> MAQILPIRFQEHLQLQNLGINPANIGFSTLTMESDKFICIREKVGEQAQVVIIDMNDPSNPIRRPISADSAIMNPASKVIALKAGKTLQIFNIEMKSKMKAHTMTDDVTFWKWISLNTVALVTDNAVYHWSMEGESQPVKMFDRHSSLAGCQIINYRTDAKQKWLLLTGISAQQNRVVGAMQLYSVDRKVSQPIEGHAASFAQFKMEGNAEESTLFCFAVRGQAGGKLHIIEVGTPPTGNQPFPKKAVDVFFPPEAQNDFPVAMQISEKHDVVFLITKYGYIHLY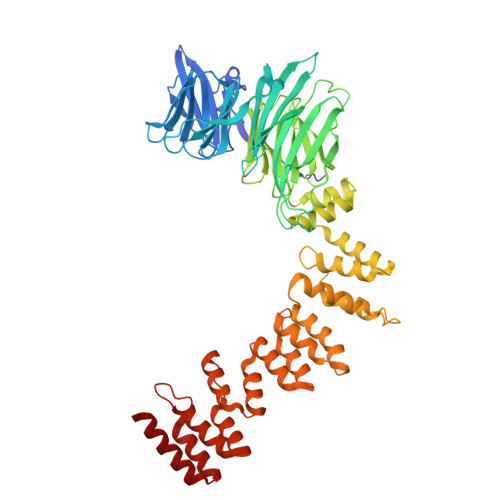DLETGTCIYMNRISGETIFVTAPHEATAGIIGVNRKGQVLSVCVEEENIIPYITNVLQNPDLALRMAVRNNLAGAEELFARKFNALFAQGNYSEAAKVAANAPKGILRTPDTIRRFQSVPAQPGQTSPLLQYFGILLDQGQLNKYESLELCRPVLQQGRKQLLEKWLKEDKLECSEELGDLVKSVDPTLALSVYLRANVPNKVIQCFAETGQVQKIVLYAKKVGYTPDWIFLLRNVMRISPDQGQQFAQMLVQDEEPLADITQIVDVFMEYNLIQQCTAFLLDALKNNR>[2x]DRLQGIVEPIVARQPLKLGVTVVHLLDNFYKGIAYGIVDEARRSNVEVVQVAVAGAYGNVQQQFAQLQSFKTLGVDYAVLSPAAYSGYDPVVADLARSGIKTISAGIPVNSDKIAFGVLQDDTLIGKVLGKALCDDGAQGKQVIVVPGAAGLEWPRLRYEGFKEVASACGAK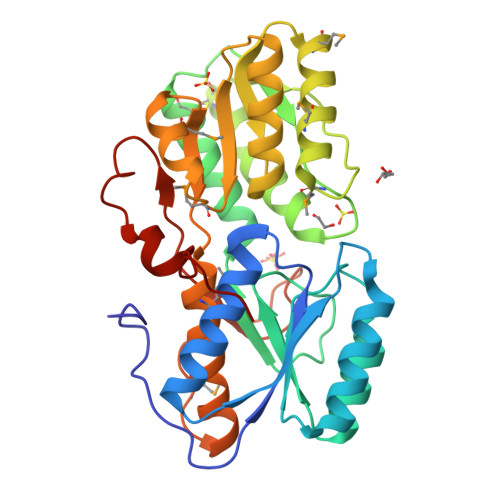LTPAAFRGEMSLADGMAQTQDLLMRTPDAEYVFTPVTFLGIGAVRAARQANRPVKVLTSAMVKENEAMIREGRLLAVASEPGVIMGRLIVQYAIREHEGLPMPPLDKPTRSVPYPHFNVPITVVDKSNVDTHPYAFYDYPPQGWSIETA1-{[5-(5-CHLORO-2-THIENYL)ISOXAZOL-3-YL]METHYL}-N-(1-ISOPROPYLPIPERIDIN-4-YL)-1H-INDOLE-2-CARBOXAMIDE 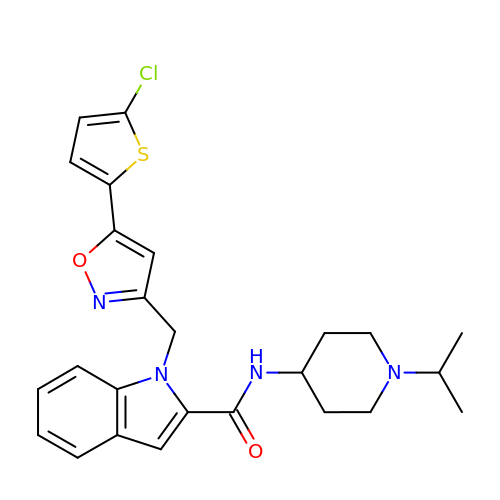| C25 H27 Cl N4 O2 S | MMGXOGPDBICRQF-UHFFFAOYSA-N> MELIGDY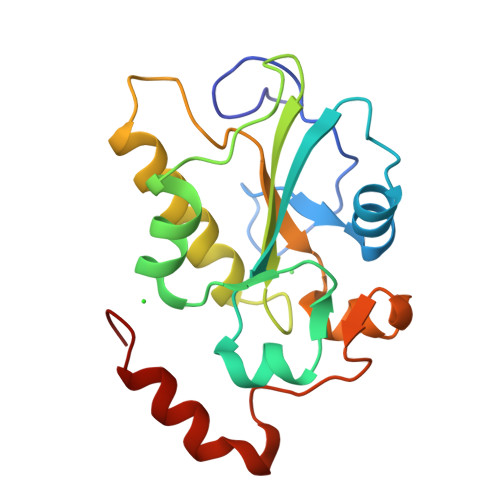SKAFLLQTVDGKHQDLKYISPETMVALLTGKFSNIVDKFVIVDCRYPYEYEGGHIKTAVNLPLERDAESFLLKSPIAPCSLDKRVILIFHDEFSSERGPRMCRFIRERDRAVNDYPSLYYPEMYILKGGYKEFFPQHPNFCEPQDYRPMNHEAFKDELKTFRLKTRSW> MHHHHHHYFSINDSKILSLQNKKNTLMDTSGYNAEVRVEGNVQLNPIFPFDFKLGSSGDDRGKVIVTQNENIVYNAMYESFSISFWIRINKWVSNLPGYTIIDSVKNNSGWSIGIISNFLVFTLKQNENSEQDINFSYDISKNAAGYNKWFFVTITTNMMGNM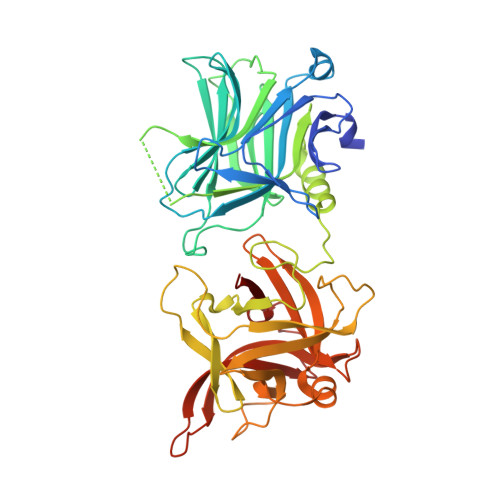MIYINGKLIDTIKVKELTGINFSKTITFQMNKIPNTGLITSDSDNINMWIRDFYIFAKELDDKDINILFNSLQYTNVVKDYWGNDLRYDKEYYMINVNYMNRYMSKKGNGIVFNTRKNNNDFNEGYKIIIKRIRGNTNDTRVRGENVLYFNTTIDNKQYSLGMYKPSRNLGTDLVPLGALDQPMDEIRKYGSFIIQPCNTFDYYASQLFLSSNATTNRLGILSIGSYSFKLGDDYWFNHEYLIPVIKIEHYASLLESTSTHWVFVPAS>MGLMNAFDSQTEDSSPAIGRNLRSRPLARKKLSEMVEEELEQMIRRREFGEGEQLPSERELMAFFNVGRPSVREALAALKRKGLVQINNGERARVSRPSADTIIGELSGMAKDFLSHPGGIAHFEQLRLFFESSLVRYAAEHATDEQIDLLAKALEINSQSLDNNAAFIRSDVDFHRVLAEIPGNPIFMAIHVALLDWLIAARPTVTDQALHEHNNVSYQQHIAIVDAIRRHDPDEADRALQSHLNSVSATWHAFG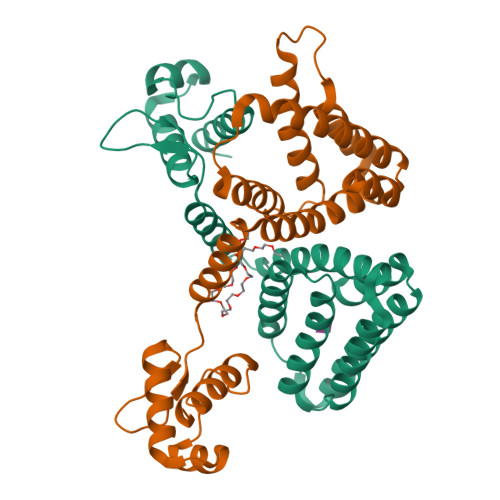QTTNKKK[2x]>AEEGAVAVCVRVRPLNSREESLGETAQVYWKTDNNVIYQVDGSKSFNFDRVFHGNETTKNVYEEIAAPIIDSAI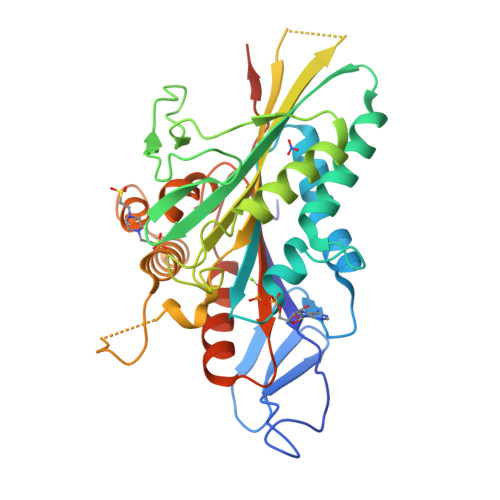QGYNGTIFAYGQTASGKTYTMMGSEDHLGVIPRAIHDIFQKIKKFPDREFLLRVSYMEIYNETITDLLCGTQKMKPLIIREDVNRNVYVADLTEEVVYTSEMALKWITKGEKSRHYGETKMNQRSSRSHTIFRMILESREKGEPSNCEGSVKVSHLNLVDLAGSERAAQTGAAGVRLKEGCNINRSLFILGQVIKKLSDGQVGGFINYRDSKLTRILQNSLGGNAKTRIICTITPVSFDETLTALQFASTAKYMKNTPYVNEVSTDELEHHHHHH[2x]>MNFFGLVGEKLSHSVSPQIHKRVFEILNIESAYKNFEISKEDISKLDGAIKLLGIQGVNVTVPYKERIMKYLDFISPEAKRIGAVNTILLRENMLYGYNTDYFGLDSMFKMANIDVQGKVAVILGTGGASKAALTYFIDSGIEKLYVSTRKKDDKKLLNSKAILIDYEELKHIKGDIILNATPVGMYPNVGISPVSKSIIQNFDILIDLIYNPGETEFLRIGNSMGKKTCDGLYMLVGQAIKSQEIWQDTKIDNSILDVIYNELKLEFLGENLY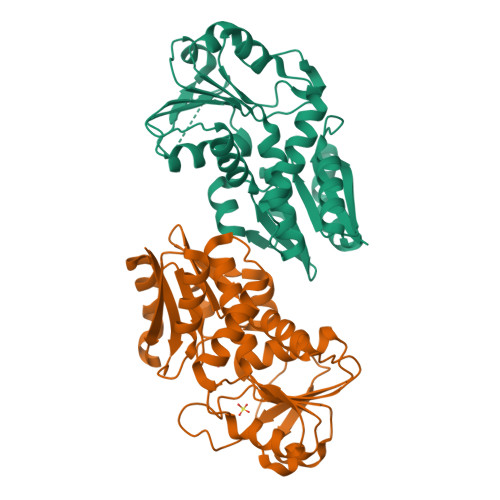FQ[2x]> MKKA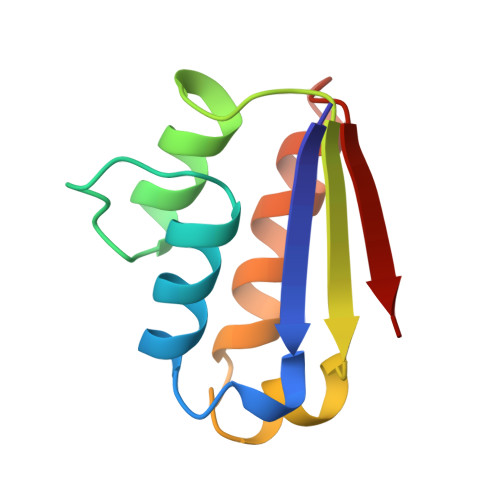VINGEQIRSISDLHQTLKKELALPEYYGENLAALWDCLTGWVEYPLVLEWRQFEQSKQLTENGAESVLQVFREAKAEGCDITIILS>SDALLVPDKCKFLHQERMDVCETHLHWHTV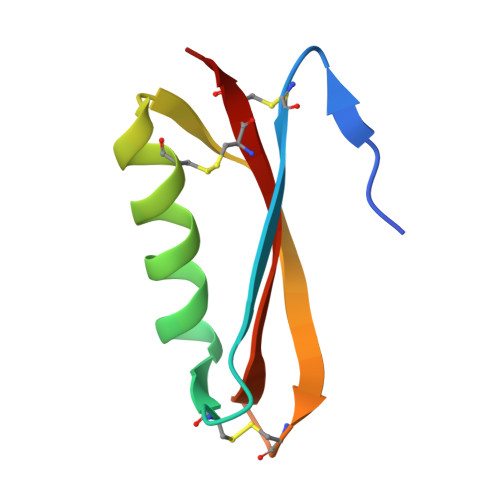AKETCSEKSTNLHDYGMLLPCGIDKFRGVEFVCCPL[2x]> MEYVKNVVCPFCGTLCDDIICKVEGNEIVGTINACRIGHSKFVHAEGAMRYKKPLIRKNGEFVEVSYDEAIDKAAKILAESKRPLMYGWSCTECEAQAVGVELAEEAGAVIDNTASVCHGPSVLALQDVGYPICTFGEVKNRADVVVYWGCNPMHAHPRHMSRNVFARGFFRERGRSDRTLIVVDPRKTDSAKLADIHLQLDFDRDYELLDAMRACLLGHEILYDEVAGVPREQIEEAVEVLKNAQFGILFFGMGITHSRGKHRNIDTAIMMVQDLNDYAKWTLIP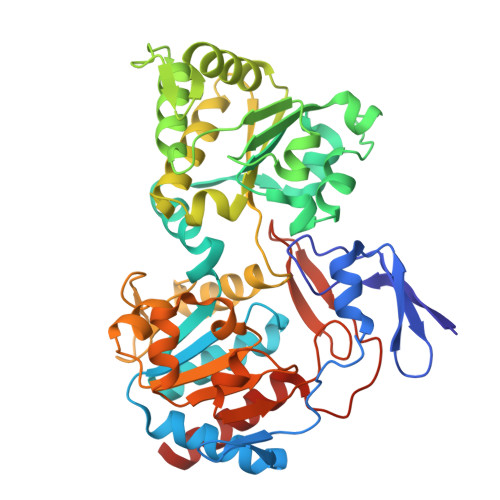MRGHYNVTGFNQVCTWESGYPYCVDFSGGEPRYNPGETGANDLLQNREADAMMVIASDPGAHFPQRALERMAEIPVIAIEPHRTPTTEMADIIIPPAIVGMEAEGTAYRMEGVPIRMKKVVDSDLLSDREILERLLEKVREYKASK>GSHMVG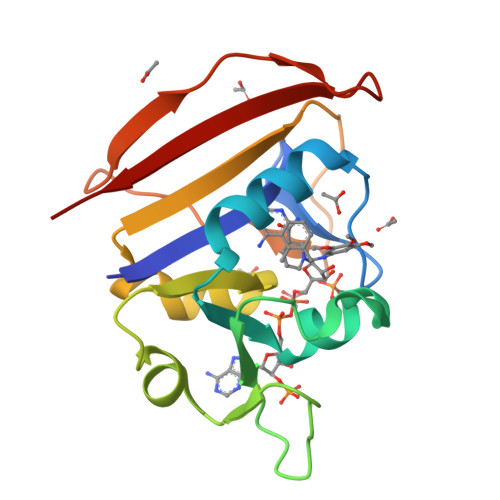LIWAQATSGVIGRGGDIPWRLPEDQAHFREITMGHTIVMGRRTWDSLPAKVRPLPGRRNVVLSRQADFMASGAEVVGSLEEALTSPETWVIGGGQVYALALPYATRCEVTEVDIGLPREAGDALAPVLDETWRGETGEWRFSRSGLRYRLYSYHRS[4x]> MKNLRYKLLLFVFIGFWGLLALNLFILSVKNQEYYEKLAERNMTKKEFLVPTRGNITDRNDEFLATNELVFGVFLPSGLKQKDLLEKIEIIQKFFPNFSKETLLNNYQKENSLYNHNLIKVVGFIPYATMQPLYAKLIQTQGIFALPLDKRYYPNNALASHVLGYVGVASLQDLKDDEENQYSQIVGKTGIEKEYNKLLQGKVGYKIMRVNALNQELATLEVVLPSTNNHLQLSLDKRLQKEADKLFENKRGAILVMDAENGELLVAGSYPEYNLNDFVGGISQDKWQKLQDDIYNPLLNRFANALYPPGSVVKMGVGLSFLENL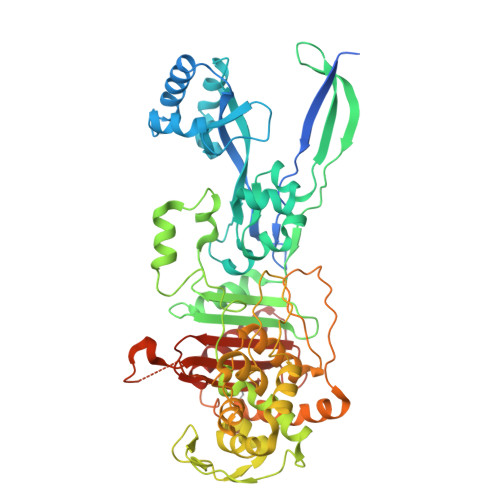HITENTTIPTPPFIEVGKHKFRDWKKTGHGNSNLYKAIRESVDVYFYKFGLEISIEKLSKTLREVGFGEKTGVDLPNEFVGIVPDNLWKLKRFNQDWRVGDTLITAIGQGSFLATPLQVLAYTGLIATGKLATPHFAINNKQPLKDPLNSFQKKKLQALRVGMYEVCNHKDGTAYHSTRGSKITLACKTGTAQVVEIAQNIVNRMKEKDMEYFHRSHAWITAFLPYEKPKYAITILVEHGEGGSKLGGLLVKMSNKLYELGYLHHHHHH> SNAPPGTVDKKMVEKCWKLMDKVVRLCQNPKLALKNSPPYILDLLPDTYQHLRTI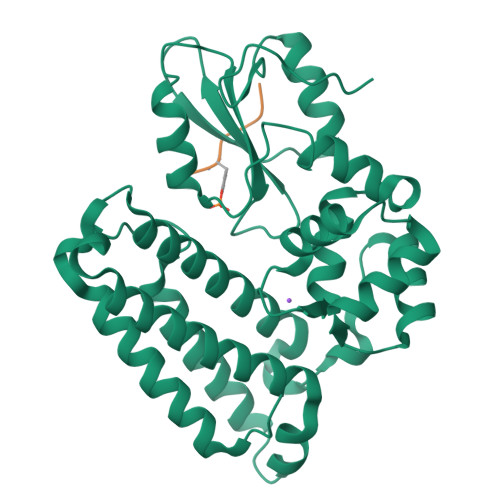LSRYEGKMETLGENEYFRVFMENLMKKTKQTISLFKEGKERMYEENSQPRRNLTKLSLIFSHMLAELKGIFPSGLFQGDTFRITKADAAEFWRKAFGEKTIVPWKSFRQALHEVHPISSGLEAMALKSTIDLTCNDYISVFEFDIFTRLFQPWSSLLRNWNSLAVTHPGYMAFLTYDEVKARLQKFIHKPGSYIFRLSCTRLGQWAIGYVTADGNILQTIPHNKPLFQALIDGFREGFYLFPDGRNQNPDLTG;> XEYTEGPT>GSMHLRPIATPYPVKEWLQPKRYKAHLMGTTYVYDFPELFRQASSSQWKNFSADVKLTDDFFISNELIEDENGELTEVEREPGANAIGMVAFKITVKTPEYPRGRQFVVVANDITFKIGSFGPQEDEFFNKVTEYARKRGIPRIYLAANSGARIGMAEEIVPLFQVAWNDAANPDKGFQYLYLTSEGMETLKKFDKENSVLTERTVINGEERFVIKTIIGSEDGLGVECLRGSGLIAGATSRAYHDIFTITLVTCRSVGIGAYLVRLGQRAIQVEGQPIILTGAPAINKMLGREVYTSNLQLGGTQIMYNNGVSHLTAVDDLAGVEKIVEWMSYVPAKRNMPVPILETKDTWDRPVDFTPTNDETYDVRWMIEGRETESGFEYGLFDKGSFFETLSGWAKGVVVGRARLGGIPLGVIGVETRTVENLIPADPANPNSAETLIQEPGQVWHPNSAFKTAQAINDFNNGEQLPMMILANWRGFSGGQRDMFNEVLKYGSFIVDALVDYKQPIIIYIPPTGELRGGSWVVVDPTINADQMEMYADVNARAGVLEPQGMVGIKFRREKLLDTMNRLDDKYRELRSQLSNKSLAPEVHQQISKQLADRERELLPIYGQISLQFADLHDRSSRMVAKGVISKELEWTEARRFFFWRLRRRLNEEYLIKRLSHQVGEASRLE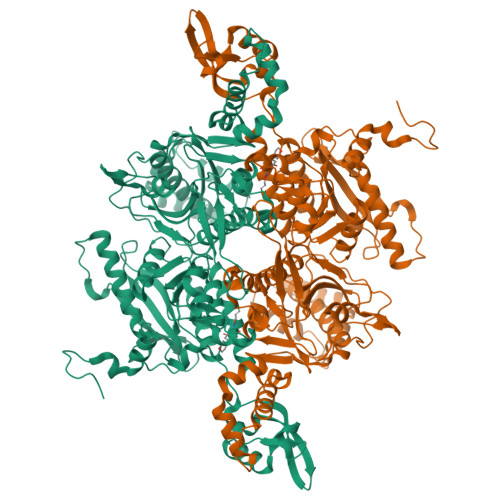KIARIRSWYPASVDHEDDRQVATWIEENYKTLDDKLKGLKLESFAQDLAKKIRSDHDNAIDGLSEVIKMLSTDDKEKLLKTLK[3x]> GAMDPRVTMNEFEYLKLLGKGTFGKVILVKEKATGRYYAMKILKKEVIVAKDEVAHTLTENRVLQNSRHPFLTALKYSFQTHDRLCFVMEYANGGELFFHLSRERVFSEDRARFYGAEIVSALDYLHSEKNVVYRDL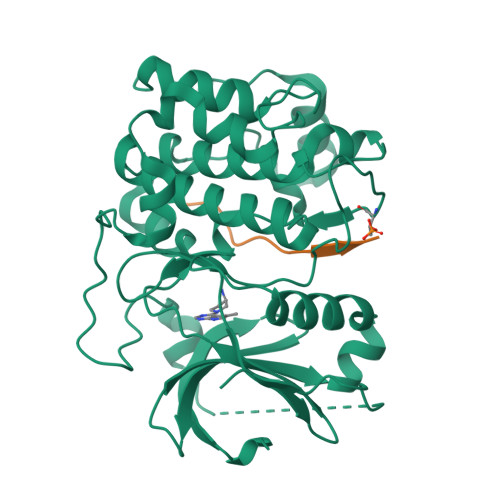KLENLMLDKDGHIKITDFGLCKEGIKDGATMKTFCGTPEYLAPEVLEDNDYGRAVDWWGLGVVMYEMMCGRLPFYNQDHEKLFELILMEEIRFPRTLGPEAKSLLSGLLKKDPKQRLGGGSEDAKEIMQHRFFAGIVWQHVYEKKLSPPFKPQVTSETDTRYFDEEFTAQMITITPPDQDDSMECVDSERRPHFPQFDYSASSTA;> GRPRTTSFAE>MPSVYGARLTTFEDEEKESEYGYVRKVSGPVVIADGMNGAAMYELVRVGHDNLIGEIIRLEGDSATIQVYEETAGLMVNDPVLRTHKPLSVELGPGILGNIFDGIQRPLKTIAIRSGDVYIPRGVSVPALDKDTLWEFQPKKIGEGDLLTGGDLYATVFENSLMQHHVALPPDAMGKVTYVAPAGQYSLKDTVLELEFQGVKKSFTMLQAWPVRTPRPVSSKLAADTPLLTGQRVLDALFPSVLGGTCAIPGAFGCGKTVISQALSKYSNSDTVVYVGCGERGNEMAEVLMDFPQLTMTLPDGREESVMKRTTLVANTSNMPVAAREASIYTGITIAEYFRDMGYNVSMMADSTSRWAEALREISGRLAEMPADSGYPAYLAARLASFYERAGKVKCLGGPERTGSVTIVGAVSPPGGDFSDPVTSATLSIVQVFWGLDKKLAQRKHFPSVNWLISYSKYSTALESFYEQFDPDFINIRTKAREVLQREDDLNEIVQLVGKDALAEGDKITLETAKLLREDYLAQNAFTPYDKFCPFYKSVWMMRNIIHFYNLANQAVEKGAGMDGQKITYTLIKHRLGDLFYRLVSQKFEDPAEGEPALVAKFKKLHEDLTAGFRALEDETR[3x];>[3x]MGVAQNNVDMEEGTLEVAMEYRTVTGVAGPLVILDKVKGPKYYEIVNIRLGDGTMRRGQVLEVDGEKAVVQVFEGTSGIDNKFTTVQFTGEVLKTPVSLDMLGRIFNGSGKPIDNGPPILPEAYLDISGSSINPSERTYPEEMIQTGISTIDVMNSIARGQKIPLFSAAGLPHNEIAAQICRQAGLVKRLEKTDNLLEDGEEDNFAIVFAAMGVNMETAQFFKRDFEENGSMERVTLFLNLANDPTIERIITPRIALTTAEYLAYECGKHVLVILTDMSSYADALREVSAAREEVPGRRGYPGYMYTDLAQIYERAGRIEGRKGSITQIPILTMPNDDITHPTPDLTGYITEGQIYIDRQLQNRQIYPPINVLPSLSRLMKSAIGEGMTRRDHSDVSNQLYANYAIGKDVQAMKAVVGEEALSSEDLLYLEFLDKFERKFVAQGAYDSRNIFQSLDLAWTLLRIFPRELLHRIPGKTLDQYYSRDAAN;>MNDADVSKQIQQMVRFIRQEAEEKANEISVSAEEEFNIEKLQLVEAEKKKIRQEYERKEKQVEIRKKIEYSMQLNASRIKVLQAQDDLVSNMMEAASKEVLNVSRDHNSYKKLLKGLIVQSLLRLKEPAVLLRCRKDDHHLVESVLESAKEEYAQKLQVHPPEIIVDHHIYLPPGPGHHNAHGPSCSGGVVVASRDGKIVCENTLDARLDVVFRKKLPEIRKQLVSQVAA[3x];>MASNRGHGGIQQLLAAEQEAQHIVAAARNAKMARLRQAKEEAEREIAEHRAQVEREFQRKLAESSGDSGANVKRLEQETEVKIHHLNAGAEKIQYDVVQMLLKHVTTVKN[3x];> MAQNQRLTVVPTVTMLGVMKSRLVGATRGHALLKKKSDALTVQFRQILKNIVTTKESMGEVMKDSSFALIEAKYVAGENIKHIVLENVQNASIKVRSRQENIAGVKIPKFEYFTDGETKNDLTGLARGGQQVQQCRAAYVKAIELLVELASLQTSFLTLDEAIKTTNRRVNALENVVKPRLENTITYIKGELDELEREDFFRLKKIQGYKKREIERQLASSKQFVEEQFAEKVSLQKGISIKSAQNLLSAGEKDEDIIF;> MAGRAQIPTKSSALIAMIADEDTVTGFLLAGVGNVDLRRKTNYLIVDSKTTVKAIEDAFKEFTTKEDIAIVLISQYVANMIRFLVDSYNKPIPAILEIPSKDHPYDPAHDSVLSRVKNLFSAESVASGRR;> MASRYWVVSLPVQNSAASVWNRLQEQISKHSFDTPLYRFNIPNLRVGTLDSLLALSDDLVKSNSFVESVSHKIRRQIEELERVSGIESSSLSVDGVPVDTYLTRFVWDEAKYPTMSPLREIVDGIHTLVAKIEDDLKVRVAEYNNVRSQLNAINRKQSGSLAVRDLSNLVKPEDIITSEHLVTLLAVVPKYSQKDWLASYETLTSYVVPRSSKLLYEDNEYALYTVTLFGRVADNFRIAAREKGFQIRDFEYSSEAQESRNQELEKLVHDQESLRSSLLQWCYTSYGEVFSSWMHFCAVRVFAESILRYGLPPSFLACVLAPSVKGEKKVRSILEELCGNANSTFWKSEDDGGMMAGLGGDADSHPYVSFTINLV;> MDHAELTTEQVLKRDIPWETYMTTKLISGTGLQLLRRYDNRSESHRAQLLDDDGPSYVRVFVSILRDIYKEETVEYVLALIDEMLTANPKRARLFHDKSLASEDTYEPFLRLLWKGNWFIQEKSCKILASIVSARPKPQDRFFANGEASNSKSKSTTIDDVLKLLVEWLCAQLKKPSHPSRGVPVAINCLAALLKEPMVRSSFVQADGVKLLTPLISPASTQQSIQLLYETCLCVWLLSYYEPAVEYLATTRTLPRLIDVVKSSTKEKVVRVVVLILRNLLPKGNFAAQMIDLGLPQVVQSLKAQAWSDEDLLEGLNQLEEGLKDNIKRLSSFDKYKQEVLLGHLDWSPMHKDPLFWRDNITNFEENDFQILRVLLTILDTSSDPRALAVACFDLSQFIQYHPAGRVIVTDLKAKERVMKLMNHENTEVTKSALLCIQRLFLGAKYASFLQA;> MAELQSGGGGGCCPPMDLFRSEPMQLVQIIIPIESAHLTVSYLGELGLLQFKDLNSEKSPFQRTYAAQIKKCAEMARKLRFFKEQMLKAGILSSVKSTTRADNNTDDLEVKLGDLEAELVEINANGDKLQRAHSELVEYKLVLQKAGEFFSSALTSAAAQQREMESQQTGEMTIETPLLTDKEMSADPSKQIKLGFIAGLVPREKSMSFERMLFRATRGNVFLRQAVVDEPVVDPVSGEKMEKNVFVVFYSGERAKNKILKICDAFGANRYPFNEEFDKQAQAISEVSGRLSELKTTLDAGLLHRGNLLQTIGDQFEQWNLLVKREKSIYHTLNMLSLDVTKKCLVGEGWSPVFATKQIQDALERAAFDSNSQVGAIFQVLHTKESPPTYFRTNKFTSAFQEIVDAYGVAKYREANPGVFTIVTFPFLFAVMFGDWGHGICLLLGTLVLIVREKKLASQKLDDITDMTFGGRYVILMMALFSIYTGLIYNEFFSVPFEIFSHSAYACRDLSCSEATTVGLIKVRDTYPFGVDPVWHGSRSELPFLNSLKMKMSILLGVAQMNLGIILSYFNATFFRIGVNIWCQ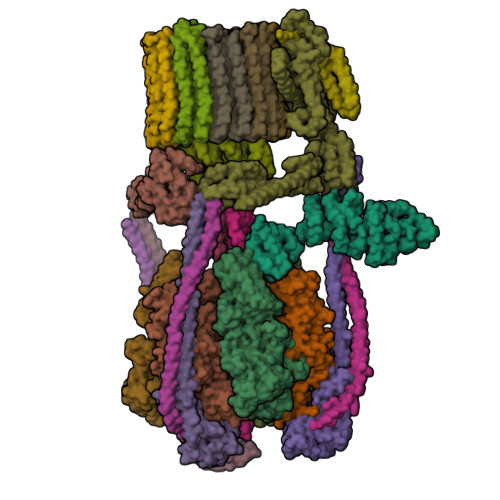FIPQIIFLNSLFGYLSLLIILKWITGSQADLYHVMIYMFLSPTDELGDNQLFPGQKTAQLVLLLLAFVSVPWMLLPKPFILKMQHQDRHQGQSYEALQSTDESLQPDTNHDSHGHEEFEFSEVFVHQMIHTIEFVLGAVSNTASYLRLWALSLAHSELSSVFYEKVLLLAWGYNNILILIVGIIVFIFATVGVLLVMETLSAFLHALRLHWVEFQNKFYEGDGYKFSPFSFALLDDEDE;> MSGSVMLGESSSWSRALVKISPYTFSAIGIAVAIGVSVLGAAWGIYITGSSLIGAAIKAPRITSKNLISVIFCEAVAIYGVIVAIILQTKLESVPASQIYAPESLRAGYAIFASGIIVGFANLVCGLCVGIIGSSCALSDAQNSSLFVKILVIEIFGSALGLFGVIVGIIMSAQASWPAKPV;> MYGFEAMTFNIHGGYLEAIVRGYRAGLLTAADYNNLCQCETLDDIKMHLSATEYGPYLQNEPSPLHTTTIVEKCTLKLVDEYKHMLCQATEPLSTFLEYITYGHMIDNVVLIVTGTLHERDVQELLEKCHPLGMFDSIATLAVAQNMRELYRLVLVDTPLAPYFSECITSEDLDDMNIEIMRNTLYKAYLEDFYKFCQKLGGATAEIMSDLLAFEADRRAVNITINSIGTELTRDDRRKLYSNFGLLYPYGHEELAVCEDIDQVRGVMEKYPPYQSIFSKLSYGESQMLDKAFYEEEVKRLCLAFEQQFHYGVFFAYMRLREQEIRNLMWISECVAQNQKSRVHDSVVFIF;> MGFLVTTLVFLVIGIIASLCTRICCNRGPSTNLLHLTLVITATVSCWMMWAIVYLAQMKPLIVPILSEEE;>MSTFSGDETAPFFGFLGAAAALVFSCMGAAYGTAKSGVGVASMGVMRPELVMKSIVPVVMAGVLGIYGLIIAVIISTGINPKAKSYYLFDGYAHLSSGLACGLAGLSAGMAIGIVGDAGVRANAQQPKLFVGMILILIFAEALALYGLIVGIILSSRAGQSRAE[9x]>[2x]GAEIYNKDGNKV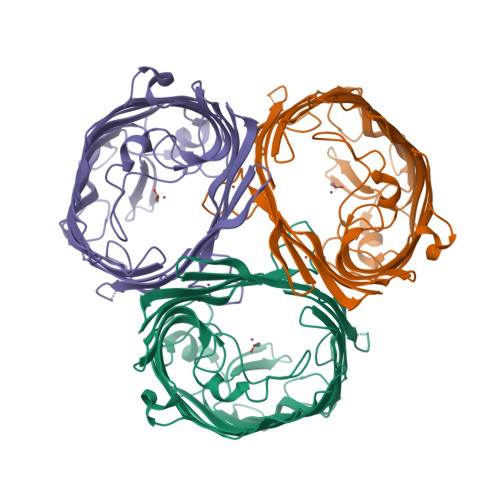DLYGKAVGLHYFSKGNGENSYGGNGDMTYARLGFKGETQINSDLTGYGQWEYNFQGNNSEGADAQTGNKTRLAFAGLKYADVGSFDYGRNYGVVYDALGYTDMLPEFGGDTAYSDDFFVGRVGGVATYRNSNFFGLVDGLNFAVQYLGKNERDTARRSNGDGVGGSISYEYEGFGIVGAYGAADRTNLQEAQPLGNGKKAEQWATGLKYDANNIYLAANYGETRNATPITNKFTNTSGFANKTQDVLLVAQYQFDFGLRPSIAYTKSKAKDVEGIGDVDLVNYFEVGATYYFNKNMSTYVDYIINQIDSDNKLGVGSDDTVAVGIVYQF> SSLDDKPQFPGASAEFIDKLEFIQPNVISGIPIYRVMDRQGQIINPSEDPHLPKEKVLKLYKSMTLLNTMDRILYESQRQGRISFYMTNYGEEGTHVGSAAALDNTDLVFGQYREAGVLMYRDYPLELFMAQCYGNISDLGKGRQMPVHYGCKERHFVTISSPLATQIPQAVGAAYAAKRANANRVVICYFGEGAASEGDAHAGFNFAATLECPIIFFCRNNGYAISTPTSEQYRGDGIAARGPGYGIMSIRVDGNDVFAVYNATKEARRRAVAENQPFLIEAMTYRIGHASTSDDSSAFRSVDEVNYWDKQDHPISRLRHYLLSQGWWDEEQEKAWRKQSRRKVMEAFEQAERKPKPNPNLLFSDVYQEMPAQLRKQQESLARHLQTYGEHYPLDHFDK;> VAHFTFQPDPEPREYGQTQKMNLFQSVTSALDNSLAKDPTAVIFGEDVAFGGVFRCTVGLRDKYGKDRVFNTPLCEQGIV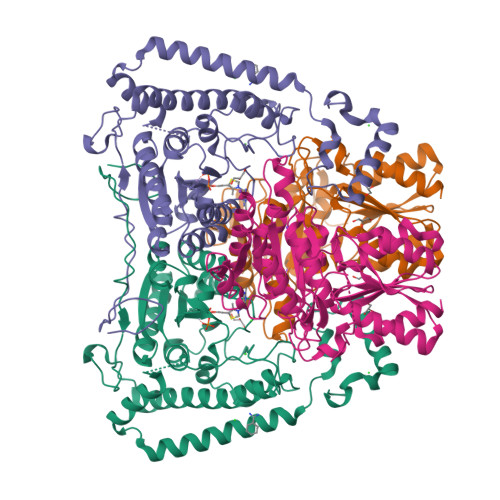GFGIGIAVTGATAIAEIQFADYIFPAFDQIVNEAAKYRYRSGDLFNCGSLTIRSPWGCVGHGALYHSQSPEAFFAHCPGIKVVIPRSPFQAKGLLLSCIEDKNPCIFFEPKILYRAAAEEVPIEPYNIPLSQAEVIQEGSDVTLVAWGTQVHVIREVASMAKEKLGVSCEVIDLRTIIPWDVDTICKSVIKTGRLLISHEAPLTGGFASEISSTVQEECFLNLEAPISRVCGYDTPFPHIFEPFYIPDKWKCYDALRKMINY(1S,2S,3S)-1-fluoranyl-2-[4-(5-fluoranylpyrimidin-2-yl)phenyl]-N-oxidanyl-3-phenyl-cyclopropane-1-carboxamide | C20 H15 F2 N3 O2 | 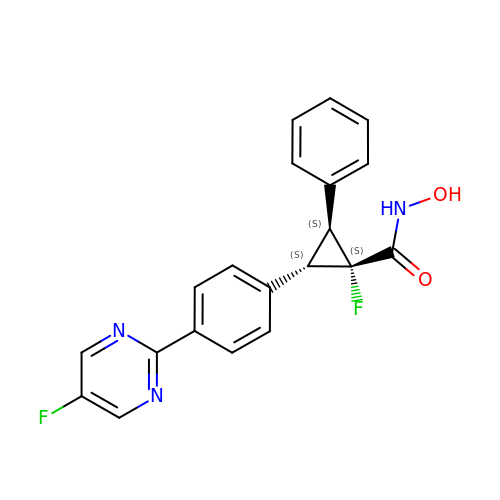MREATSZIGJDNKB-HLIPFELVSA-N> GPEFEAAACKKYMSKLRTIVAAQSRFLSTYDGAENLCLEDIYTENTLEVRTEVGMAGPLHKSPAALGLEELFSPNGHLNEDADTVLVVGEAGSGKSTLLQQVHLLWATG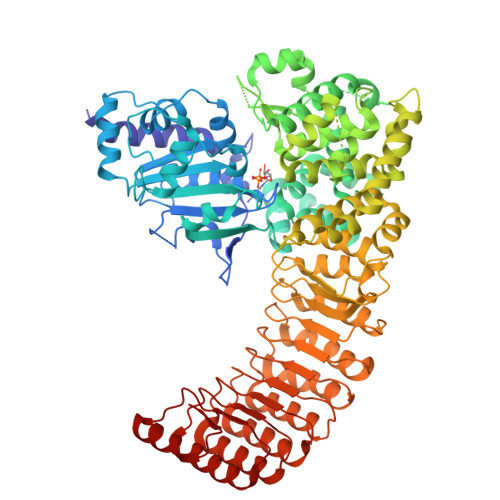QDFQEFLFVFPFSCRQLQCVARPLSVMTLLFEHCCWPDVGQQDVFQFLLDHPDRILLTFDGFDEFKFKFTDHERHCSPTDPTSVQTLLFNLLQGNLLKNARKVLTSRPDAVSAFLRKYVRTEFNLKGFSEEGIELYLRKCHREPGVADRLIHLLQTTSALHGLCHLPVFSWMVSKCHQELLLQDGGSPKTTTDMYLLILQHFLRHASLPDSASQGLGPSLLQGRLPTLLRLGQLALWGLGMCCYVFSAQQLQAAQVDPDDISLGFLVQAQGVVPGSTAPLEFLHITFQCFLAAFYLVLSTDVPTASLRYLFNCRRPGSSPLSRLLPRLCVQGSEHKESTVAALLQKTEPHNLQITAAFLAGLLSREHRDLLAACQASERSLLRRRACARWCLARSLHKHFRSIPPAVPGEAKSMHAMPGFLWLIRSLYEMQEERLAQEAVRGLNVEHLKLTFCGVGPAECAALAFVLRHLRRPVALQLDHNSVGDIGVEQLLPCLGACKALYLRDNNISDRGICKLIEHALHCEQLQKLALFNNKLTDGCAHSVAQLLACKQNFLALRLGNNHITAEGAQVLAEGLRDNSSLQFLGFWGNKVGDKGAQALAEALSDHQSLKWLSLVGNNIGSVGAQALASMLEKNVALEELCLEENHLQDAGVCSLAEGLKRNSSLKVLKLSNNCITFVGAEALLQALASNDTILEVWLRGNPFSPEEMEALSHRDSRLLL>HHHMRVSFMVAMDENRVIGKDNNLPWRLPSELQYVKKTTMGHPLIMGRKNYEAIGRPLPGRRNIIVTRNEGYHVEGCEVAHSVEEVFELCKNEEEIFIFGGAQIYDLFLPYVDKLYITKIHHAFEGDTFFPEMDMTNWKEVFVEKGLTDEKNPY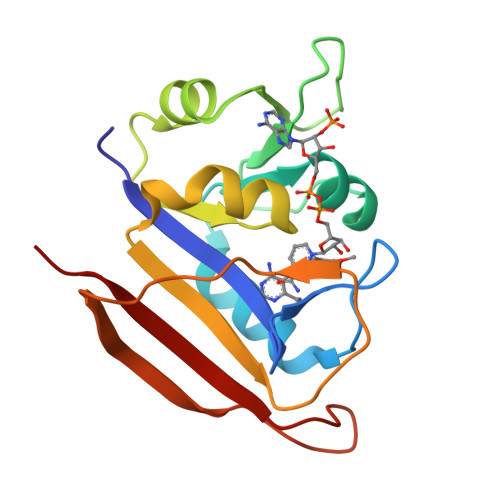TYYYHVYEKQQ[2x]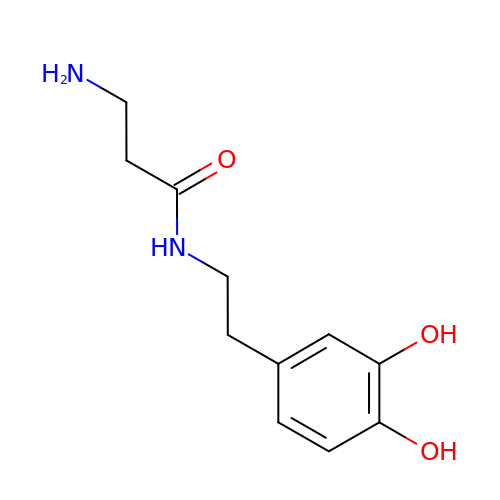N-[2-(3,4-dihydroxyphenyl)ethyl]-beta-alaninamide | C11 H16 N2 O3 | KGZWXTYWZFMLSQ-UHFFFAOYSA-N>[2x]SNAGKNVMVEPHRHEGVFICRGKEDALVTKNLVPGESVYGEKRVSISEGDDKIEYRAWNPFRSKLAAAILGGVDQIHIKPGAKVLYLGAASGTTVSHVSDIVGPDG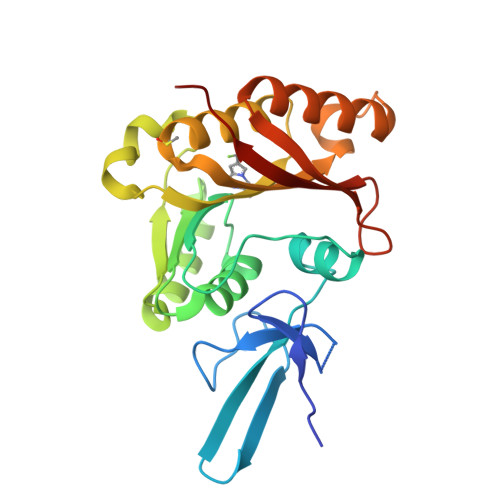LVYAVEFSHRSGRDLINLAKKRTNIIPVIEDARHPHKYRMLIAMVDVIFADVAQPDQTRIVALNAHTFLRNGGHFVISIKANCIDSTASAEAVFASEVKKMQQENMKPQEQLTLEPYERDHAVVVGVYRPPPKVKN>[8x]GSLAPMFERLSTESVQEQLPYSVTLISMPATTEGRRGFSVSVESASSNYATTVQVKEVNRMHISPNNRNAIHPGDRILEINGTPVRTLRVEEVEDAISQTSQTLQLLIEHDPVSQRLDQLRLE

LIM domain kinases (LIMK) are important regulators of actin cytoskeletal remodeling. These protein kinases phosphorylate the actin depolymerizing factor cofilin to suppress filament severing, and are key nodes between Rho GTPase cascades and actin. LIMKs across species have a common architecture, with two N-terminal tandem-zinc finger LIM domains followed by a PDZ domain, a predicted unstructured region enriched in serine, proline and glycine residues, and a C-terminal kinase domain. The LIMK PDZ domain is unusual however in that it does not interact tightly with carboxy-terminal peptides.

We expressed, purified, and crystallized the human LIMK2 PDZ domain (residues 145-236), which is monomeric in solution, and determined its structure to 2.0 Å resolution. The crystal structure revealed a compact globular domain resembling a partially open barrel that is typical of the PDZ fold. We observed the expected canonical six β-strands and the canonical αB helix, but unusually, found that helix αA is replaced by two 310 helices, which we term αA’ (residues R187-H189) and αA” (residues P192-N194). In addition, we found a third 310 helix in the βD-αB loop that we term the αB’ helix (residues V212-T214) (secondary structure nomenclature as per). We observed good electron density throughout the structure and that crystal packing appeared to induce a conformational movement in the βB-βC loop resulting in two orientations visible in the asymmetric unit. Instead, they harbor KRGL and RRGL sequences in LIMK1 and LIMK2 respectively, replacing the first hydrophobic residue with a conserved arginine residue, Arg163. Unusually for a charged residue, we found Arg163 in a similar orientation. It caps helix αB, hydrogen bonds to the carboxyl oxygens of residues Ala223, Ile224 and Gln226, and also hydrogen bonds to the carboxyl oxygen of Gln229 within the αB-βF loop. This arrangement seems to provide a rigid anchor for the C-terminus of the αB helix. In addition, an inward orientation of helix αB and placement of Arg163’s Cβ atom to encroach on the expected carboxylate binding site provides a potential explanation for why the LIMK PDZ domains do not interact with carboxy-terminal peptides with measured affinities in a biological range.> SLDGTGWN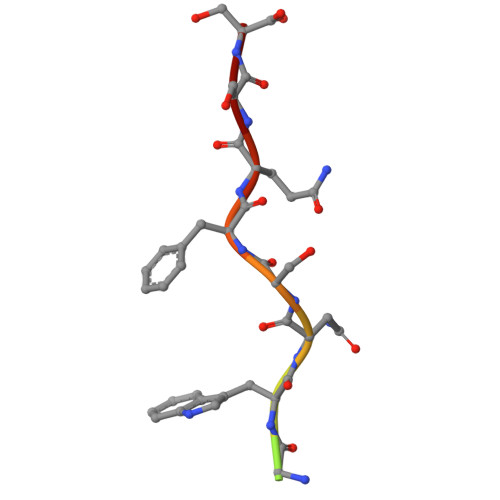SFQSS>HPETLVKVKDAEDQLGARVGYIELDLNSGKILESFRPEERFPMMSTFKVLLCGAVLSRVDAGQEQLGRRIHYSQNDLVKYSPVTEKHLTDGMTVRELCSAAITMSDN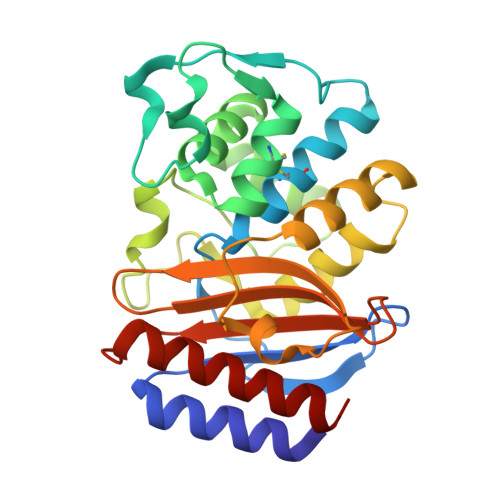TAANLLLTTIGGPKELTAFLHNMGDHVTRLDRWEPELNEAIPNDERDTTTPAAMATTLRKLLTGELLTLASRQQLIDWMEADKVAGPLLRSALPAGWFIADKSGASERGSRGIIAALGPDGKPSRIVVIYTTGSQATMDERNRQIAEIGASLIKHW[6x]> MMTTMNVLGTPLECCCQNPLTGFYRDGFCRTGAGDVGAHVVCAQMTAEFLTFTRSRGNDL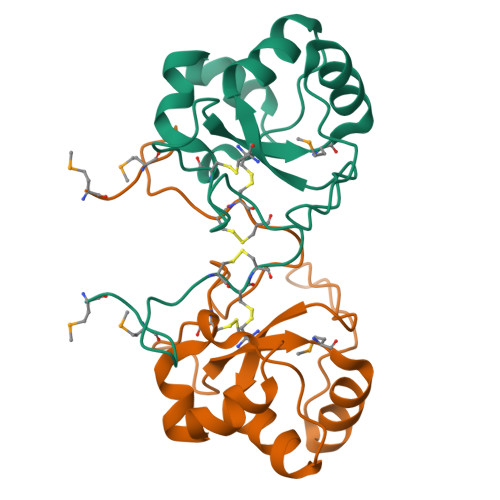STPVPAYQFPGLKPGDRWCLCASRWREALEAGVAPPVILEATHASALEYVSLEDLKAHALGGNQQRLEHHHHHH> MESHVKYLDELILAIKDLNSGVDSKVQIKKVPTDPSSSQEYAKSLKILNTLIRNLKDQRRNNIMKNDTIFSKTVSALALLLEYNPFLLVMKDSNGNFEIQRLIDDFLNISVLNYDNYHRIWFMRRKLGSWCKACVEFYGKPAKFQLTAHFENTMNLYEQALTEVLLGKTELLKFYDTLKGLYILLYWFTSEYSTFGNSIAFLDSSLGFTKFDFNFQRLIRIVLYVFDSCELAALEYAEIQLKYISLVVDYVCNRTISTALDAPALVCCEQLKFVLTTMHHFLDNKYGLLDNDPTMAKGILRLYSLCISNDFSKCFVDHFPIDQWADFSQSEHFPFTQLTNKALSIVYFDLKRRSLPVEALKYDNKFNIWVYQSEPDSSLKNVTSPFDDRYKQLEKLRLLVLKKFNKTERGTLLKYRVNQLSPGFFQRAGNDFKLILNEASVSIQTCFKTNNITRLTSWTVILGRLACLESEKFSGTLPNSTKDMDNWYVCHLCDIEKTGNPFVRINPNRPEAAGKSEIFRILHSNFLSHPNIDEFSESLLSGILFSLHRIFSHFQPPKLTDGNGQINKSFKLVQKCFMNSNRYLRLLSTRIIPLFNISDSHNSEDEHTATLIKFLQSQKLPVVKENLVIAWTQLTLTTSNDVFDTLLLKLIDIFNSDDYSLRIMMTLQIKNMAKILKKTPYQLLSPILPVLLRQLGKNLVERKVGFQNLIELLGYSSKTILDIFQRYIIPYAIIQYKSDVLSEIAKIMCDGDTSLINQMKVNLLKKNSRQIFAVALVKHGLFSLDILETLFLNRAPTFDKGYITAYLPDYKTLAEITKLYKNSVTKDASDSENANMILCSLRFLITNFEKDKRHGSKYKNINNWTDDQEQAFQKKLQDNILGIFQVFSSDIHDVEGRTTYYEKLRVINGISFLIIYAPKKSIISALAQISICLQTGLGLKEVRYEAFRCWHLLVRHLNDEELSTVIDSLIAFILQKWSEFNGKLRNIVYSILDTLIKEKSDLILKLKPYTTLALVGKPELGILARDGQFARMVNKIRSTTDLIPIFANNLKSSNKYVINQNLDDIEVYLRRKQTERSIDFTPKKVGQTSDITLVLGALLDTSHKFRNLDKDLCEKCAKCISMIGVLDVTKHEFKRTTYSENEVYDLNDSVQTIKFLIWVINDILVPAFWQSENPSKQLFVALVIQESLKYCGLSSESWDMNHKELYPNEAKLWEKFNSVSKTTIYPLLSSLYLAQSWKEYVPLKYPSNNFKEGYKIWVKRFTLDLLKTGTTENHPLHVFSSLIREDDGSLSNFLLPYISLDIIIKAEKGTPYADILNGIIIEFDSIFTCNLEGMNNLQVDSLRMCYESIFRVFEYCKKWATEFKQNYSKLHGTFIIKDTKTTNMLLRIDEFLRTTPSDLLAQRSLETDSFERSALYLEQCYRQNPHDKNQNGQLLKNLQITYEEIGDIDSLDGVLRTFATGNLVSKIEELQYSENWKLAQDCFNVLGKFSDDPKTTTRMLKSMYDHQLYSQIISNSSFHSSDGKISLSPDVKEWYSIGLEAANLEGNVQTLKNWVEQIESLRNIDDREVLLQYNIAKALIAISNEDPLRTQKYIHNSFRLIGTNFITSSKETTLLKKQNLLMKLHSLYDLSFLSSAKDKFEYKSNTTILDYRMERIGADFVPNHYILSMRKSFDQLKMNEQADADLGKTFFTLAQLARNNARLDIASESLMHCLERRLPQAELEFAEILWKQGENDRALKIVQEIHEKYQENSSVNARDRAA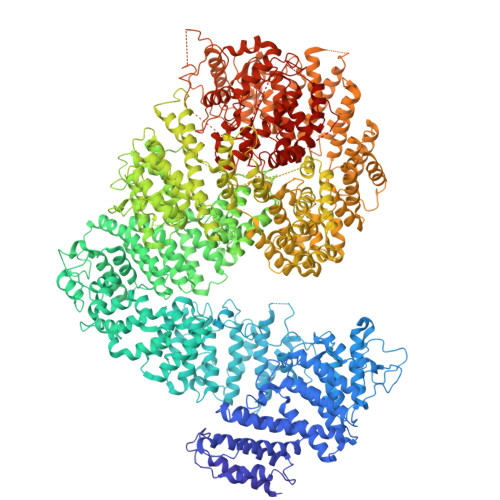VLLKFTEWLDLSNNSASEQIIKQYQDIFQIDSKWDKPYYSIGLYYSRLLERKKAEGYITNGRFEYRAISYFLLAFEKNTAKVRENLPKVITFWLDIAAASISEAPGNRKEMLSKATEDICSHVEEALQHCPTYIWYFVLTQLLSRLLHSHQSSAQIIMHILLSLAVEYPSHILWYITALVNSNSSKRVLRGKHILEKYRQHSQNPHDLVSSALDLTKALTRVCLQDVKSITSRSGKSLEKDFKFDMNVAPSAMVVPVRKNLDIISPLESNSMRGYQPFRPVVSIIRFGSSYKVFSSLKKPKQLNIIGSDGNIYGIMCKKEDVRQDNQYMQFATTMDFLLSKDIASRKRSLGINIYSVLSLREDCGILEMVPNVVTLRSILSTKYESLKIKYSLKSLHDRWQHTAVDGKLEFYMEQVDKFPPILYQWFLENFPDPINWFNARNTYARSYAVMAMVGHILGLGDRHCENILLDIQTGKVLHVDFDCLFEKGKRLPVPEIVPFRLTPNLLDALGIIGTEGTFKKSSEVTLALMRKNEVALMNVIETIMYDRNMDHSIQKALKVLRNKIRGIDPQDGLVLSVAGQTETLIQEATSEDNLSKMYIGWLPFW>[12x]MATVTATTKVPEIRDVTRIERIGAHSHIRGLGLDDALEPRQASQGMVGQLAARRAAGVVLEMIREGKIAGRAVLIAGQPGTG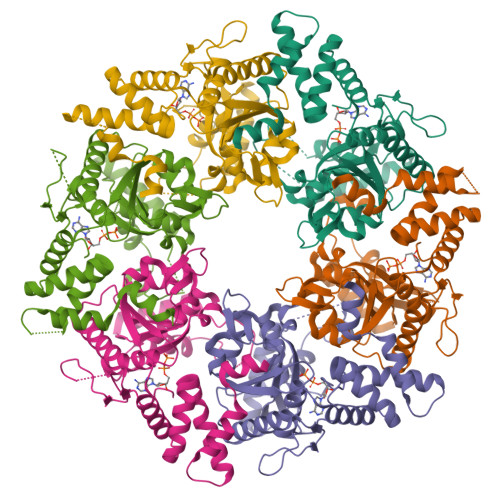KTAIAMGMAQALGPDTPFTAIAGSEIFSLEMSKTEALTQAFRRSIGVRIKAGAVHTVSLHEIDVINSRTQGFLALFSGDTGEIKSEVREQINAKVAEWREEGKAEIIPGVLFIDEVHMLDIESFSFLNRALESDMAPVLIMATNRGITRIRGTSYQSPHGIPIDLLDRLLIVSTTPYSEKDTKQILRIRCEEEDVEMSEDAYTVLTRIGLETSLRYAIQLITAASLVCRKRKGTEVQVDDIKRVYSLFLDESRSTQYMKEYQDAFLFNELKGETMDTSLEHHHHHH>[2x]MHHHH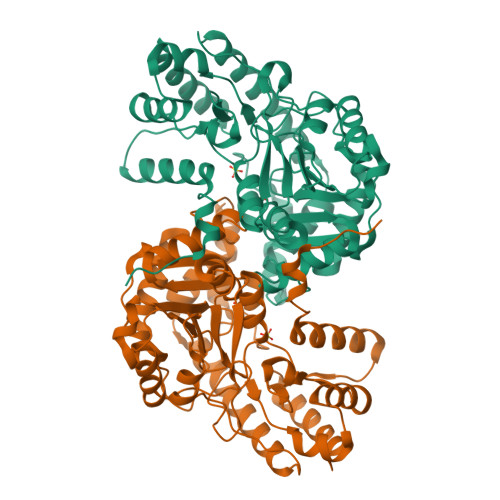HHMDIALAKRVQKVKPSPTLAVAAKAAQMKAQGLDIIGLGTGEPDFDTPQHIKLAAISAIEAGDTKYTAVDGIVELKEAVKNKFKRDNELDYQLNQILVSVGGKQSCYNLCQAYLNPGDEVIIPAPYWVSYPDMVLLADGVPVIIETTPAQRYKINAQQLEQAITPKTRMIFLNSPSNPSGIAYTQNELKELGDVLKKHPQILIATDDMYEHIIWSQPFTNILNACPELYDRTIVLNGVSKAYAMTGWRIGYAAGPAPLINAMKTIQSQSTSNPCSIAQRAAVAALNGSNESIEEMVNAFHQRHDYVADRLQSIDGIEVIPADGTFYIFPSVQAIIEKRGYANDIEFSEKLLNEVGVALVPGSAFGTEGCIRISFATGIDTLKDALNRLQRFCS> MQNKLASGARLGRQALLFPLCLVLYEFSTYIGNDMIQP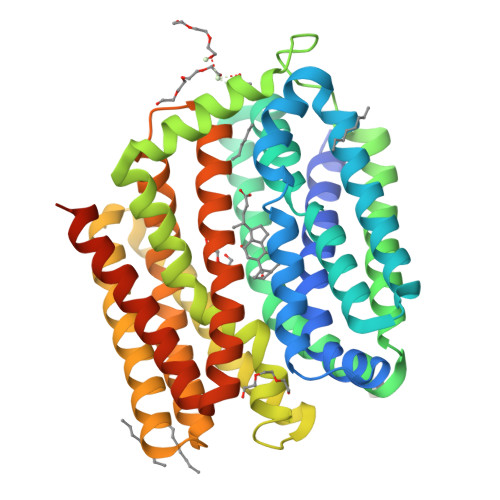GMLAVVEQYQAGIDWVPTSMTAYLAGGMFLQWLLGPLSDRIGRRPVMLAGVVWFIVTCLAILLAQNIEQFTLLRFLQGISLCFIGAVGYAAIRESFEEAVCIKITALMANVALIAPLLGPLVGAAWIHVLPWEGMFVLFAALAAISFFGLQRAMPETATRIGEKLSLKELGRDYKLVLKNGRFVAGALALGFVSLPLLAWIAQSPIIIITGEQLSSYEYGLLQVPIFGALIAGNLLLARLTSRRTVRSLIIMGGWPIMIGLLVAAAATVISSHAYLWMTAGLSIYAFGIGLANAGLVRLTEFASDMSKGTVSAAMGMLQMLIFTVGIEISKHAWLNGGNGLFNLFNLVNGILWLSLMVIFLKDKQMGNSHEGASTHHHHHH> MNVIAILNHMGVYFKEEPIRELHRALERLNFQIVYPNDRDDLLKLIENNARLCGVIFDWDKYNLELCEEISKMNENLPLYAFANTYSTLDVSLNDLRLQISFFEYALGAAEDIANKIKQTTDEYINTILPPLTKALFKYVREGKYTFCTPGHMGGTAFQKSPVGSLFYDFFGPNTMKSDISISVSELGSLLDHSGPHKEAEQYIARVFNADRSYMVTNGTSTANKIVGMYSAPAGSTILIDRNCHKSLTHLMMMSDVTPIYFRPTRNAYGILGGIPQSEFQHATIAKRVKETPNATWPVHAVITNSTYDGLLYNTDFIKKTLDVKSIHFDSAWVPYTNFSPIYEGKCGMSGGRVEGKVIYETQSTHKLLAAFSQASMIHVKGDVNEETFNEAYMMHTTTSPHYGIVASTETAAAMMKGNAGKRLINGSIERAIKFRKEIKRLRTESDGWFFDVWQPDHIDTTECWPLRSDSTWHGFKNIDNEHMYLDPIKVTLLTPGMEKDGTMSDFGIPASIVAKYLDEHGIVVEKTGPYNLLFLFSIGIDKTKALSLLRALTDFKRAFDLNLRVKNMLPSLYREDPEFYENMRIQELAQNIHKLIVHHNLPDLMYRAFEVLPTMVMTPYAAFQKELHGMTEEVYLDEMVGRINANMILPYPPGVPLVMPGEMITEESRPVLEFLQMLCEIGAHYPGFETDIHGAYRQADGRYTVKVLKE;> DKTALTVIRLGGIFSRRQQYQLPVNVTASTLTLLLQKPLKLHDMEVVHISFERSALEQWLSKGGEIRGKLNGIGFAQKLNLEVDSAQHLVVRDVSLQGSTLALPGS

extracellular pH, and works in conjunction with a cognate inner membrane antiporter. excreted by the antiporter in exchange for a new amino acid substrate. that it is a decamer made of two pentameric rings. central pore, with the CTDs at the periphery.

(cryoEM) and combined it with the crystal structures of the individual proteins. and the C-terminal β-sheet of LdcI23. 7.5 Å to 6.2 Å resolution. interacted with LdcI but was not capable of binding to LdcC. whole upon enzyme activation by pH and the binding of LARA. to the incorporation of the LdcI decamer into the LdcI-RavA cage. decameric state upon activation and incorporation into the LdcI-RavA cage.>[6x]MKNIRNFSIIAHIDHGKSTLSDRIIQICGGLSDREMEAQVLDSMDLERERGITIKAQSVTLDYKASDGETYQLNFIDTPGHVDFSYEVSRSLAACEGALLVVDAGQGVEAQTLANCYTAMEMDLEVVPVLNKIDLPAADPERVAEEIEDIVGIDATDAVRCSAKTGVGVQDVLERLVRDIPPPEGDPEGPL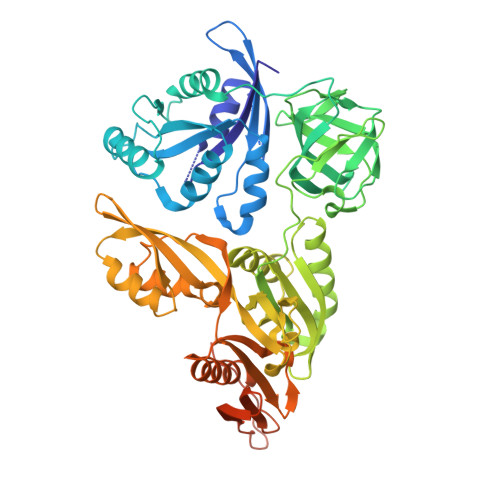QALIIDSWFDNYLGVVSLIRIKNGTLRKGDKVKVMSTGQTYNADRLGIFTPKQVDRTELKCGEVGWLVCAIKDIHGAPVGDTLTLARNPAEKALPGFKKVKPQVYAGLFPVSSDDYEAFRDALGKLSLNDASLFYEPESSSALGFGFRCGFLGLLHMEIIQERLEREYDLDLITTAPTVVYEVETTSREVIYVDSPSKLPAVNNIYELREPIAECHMLLPQAYLGNVITLCVEKRGVQTNMVYHGNQVALTYEIPMAEVVLDFFDRLKSTSRGYASLDYNFKRFQASDMVRVDVLINGERVDALALITHRDNSQNRGRELVEKMKDLIPRQQFDIAIQAAIGTHIIARSTVKQLRKNVLAKCYGGDISRKKKLLQKQKEGKKRMKQIGNVELPQEAFLAILHVGKDNK>GSMSLKPFTYPFPETRFLHAGPNVYKFKIRYGKSIRGEEIENKEVITQELEDSVRVVLGNLDNLQPFATEHFIVFPYKSKWERVSHLKFKHGEIILIPYPFVFTLYVE[2x];>GSMPVNNMVTGYISIDAMKKFLGELHDFIPGTSGYLAYHVQNE[2x]

In mammals, meiotic telomere attachments are achieved by a meiosis-specific complex of MAJIN, TERB1 and TERB2 (herein referred to as the meiotic telomere complex) that repurposes and integrates the functions of two complexes, LINC and shelterin, which otherwise perform distinct critical roles outwith meiosis. MAJIN provides the inner nuclear membrane attachment through a transmembrane helix at its C-terminus, whilst TERB1 is proposed to interact with SUN1 and cohesin components through its N-terminal armadillo repeat domain and C-terminal MYB domain, respectively. MAJIN and TERB1 are physically linked by TERB2, which binds MAJIN through its C-terminus and TERB1 through its N-terminus. Here, we report the crystal structure of the MAJIN–TERB2 complex, revealing a 2:2 heterotetramer in which two TERB2 chains wrap around a core MAJIN globular dimer.

Using this as a model for molecular replacement, we proceeded to solve the structure of a truncated complex (MAJIN 1–106 and TERB2 168–207) in an alternative crystal form at 1.85 Å resolution. Both structures are essentially the same and the subsequent discussion is based on the latter higher resolution crystal form. The MAJIN–TERB2 structure demonstrates a 2:2 heterotetrameric assembly, in which two TERB2 chains wrap around the surface of a core globular MAJIN dimer. Size exclusion chromatography small-angle X-ray scattering (SEC-SAXS) revealed scattering curves and ab initio envelopes that closely match the heterotetrameric crystal structure for the truncated construct, with the wider complex demonstrating an elongation consistent with its additional sequence being largely unstructured in solution. The MAJIN protomers adopt a β-grasp fold, in which a β-sheet grasps around a core α-helix in a β(2)-α-β(3) configuration. The five-stranded grasping β-sheet contains an insertion between β4 and β7 strands, which forms a two-stranded β-sheet appendage that splays from the base of the structure. TERB2 chains follow a meandering path from their N-termini at the MAJIN dimer interface, passing around the α-helix to complete its closure and providing an additional short β-strand to the grasping β-sheet, and terminate by forming a third β-strand of the MAJIN β-sheet appendage. This interaction is mediated largely through the insertion of hydrophobic side-chains of TERB2 into pockets on the MAJIN molecular surface, in addition to a salt bridge between MAJIN residue R14 and TERB2 residue D191, and the aforementioned β-sheet interactions. At its N-terminal end, TERB2 residue Y176 contributes to the MAJIN dimer interface that contains a hydrophobic core formed of highly conserved MAJIN residues P64, F73 and Y75. Whilst the 2:2 assembly is stable across a range of concentrations and chemical conditions, with smaller oligomers never observed in vitro, its disruption through MAJIN mutation F73E Y75E yielded a stable 1:1 complex with secondary structure composition matching that of a single MAJIN–TERB2 protomer.> GSKAPPTFKVSLMDQSVREGQDVIMSIRVQGEPKPVVS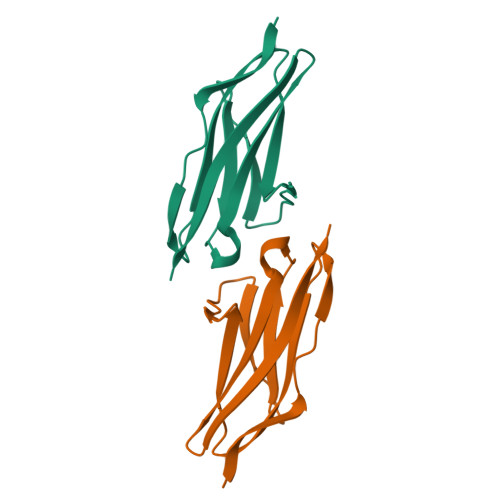WLRNRQPVRPDQRRFAEEAEGGLCRLRILAAERGDAGFYTCKAVNEYGARQCEARLEVRGE> GAMVDTLSGLSSEQGQSGDMTIEEDSATHIKFSKRDIDGKELAGATMELRDSSGKTISTWISDGQVKDFYLMPGKYTFVETAAPDGYEVATAITFTVNEQGQVTVNGKAT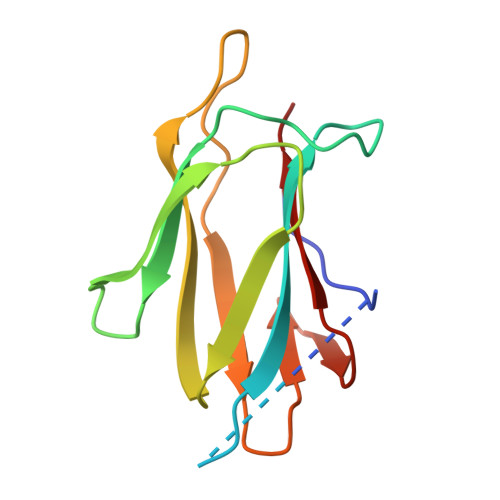KGDAHIVMVDA>LTQELGTAFFQQQQLPAAMADTFLEHLCLLDIDSEPVAARSTSIIATIGPASRSVERLKEMIKAGMNIARLNFSHGSHEYHAESIANVREAVESFAGSPLSYRPVAIALDTKGPEIRTGILQGGPESEVELVKGSQVLVTVDPAFRTRGNANTVWVDYPNIVRVVPVGGRIYIDDGLISLVVQKIGPEGLVTQVENGGVLGSRKGVNLPGAQVDLPGLSEQDVRDLRFGVEHGVDIVFASFVRKASDVAAVRAALGPEGHGIKIISKIENHEGVKRFDE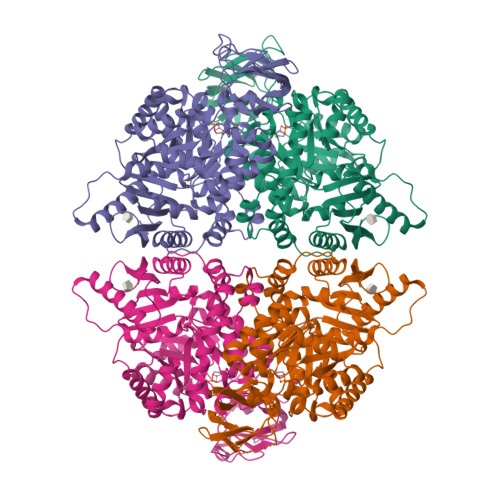ILEVSDGIMVARGDLGIEIPAEKVFLAQKMMIGRCNLAGKPVVCATQMLESMITKPRPMRAETSDVANAVLDGADCIMLSGETAKGNFPVEAVKMQHAIAREAEAAVYHRQLFEELRRAAPLSRDPTEVTAIGAVEAAFKCCAAAIIVLTTTGRSAQLLSRYRPRAAVIAVTRSAQAARQVHLCRGVFPLLYREPPEAIWADDVDRRVQFGIESGKLRGFLRVGDLVIVVTGWRPGSGYTNIMRVLSIS[4x]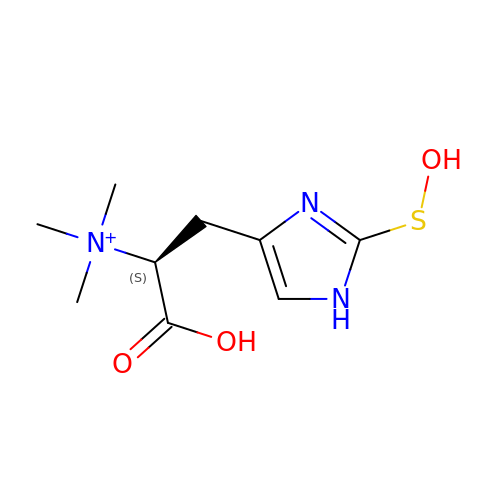(1S)-1-carboxy-2-[2-(hydroxysulfanyl)-1H-imidazol-4-yl]-N,N,N-trimethylethan-1-aminium | C9 H16 N3 O3 S | ZLPHHLCGSBYNCO-ZETCQYMHSA-O>GHMNDALHIGLPPFLVQANNEPRVLAAPEARMGYVLELVRANIAADGGPFAAAVFERDSGLLIAAGTNRVVPGRCSAAHAEILALSLAQAKLDTHDLSADGLPACELVTSAEPCVMCFGAVIWSGVRSLV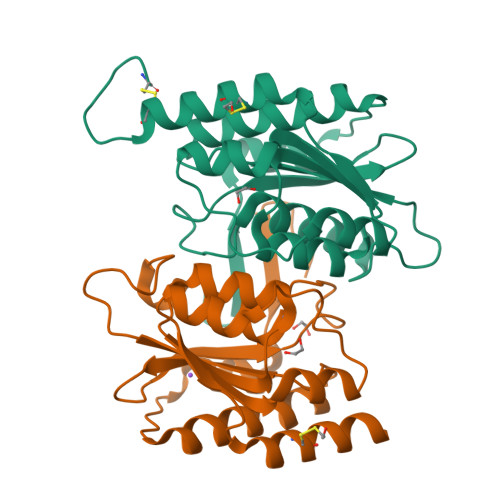CAARSDDVEAIGFDEGPRPENWMGGLEARGITVTTGLLRDAACALLREYNACNGVIYNARCGVHKGS[2x]~{N}-[(2~{S})-2-morpholin-4-ylpropyl]-4-oxidanylidene-3,5-dihydro-2~{H}-1,5-benzothiazepine-7-carboxamide | C17 H23 N3 O3 S | 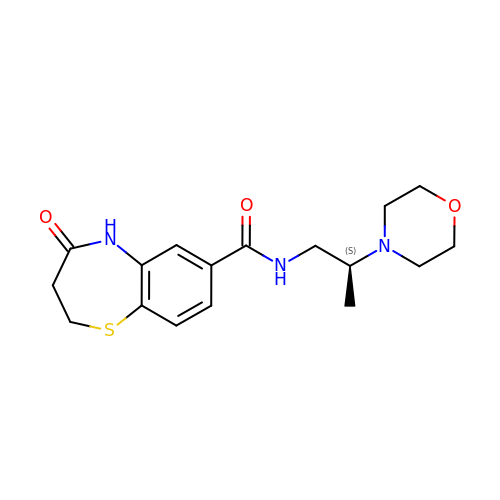MNYMDWGPOVDYSU-LBPRGKRZSA-N> KFNDTLFGEMLHGYNNRTQHVNQGQVFQMTFRENNFIKDFPQLADGLLVIPLPVEEQCRGVLSEPLPDLQLLTGDIRYDEAMGYPMVQQWRVRSNLYRVKLSTITLAAGFTNVLKILTKESSREELLSFIQHYGSHYIAEALYGSELTCIIHFPSKKVQQQLWLQYQKETTELGSKKELKSMPFITYLSGLLTAQMLSDDQLISGVEIRCEEKGRCPSTCHLCRRPGKEQLSPTPVLLEINRVVPLYTLIQDNGTKEAFKSALMSSYWCS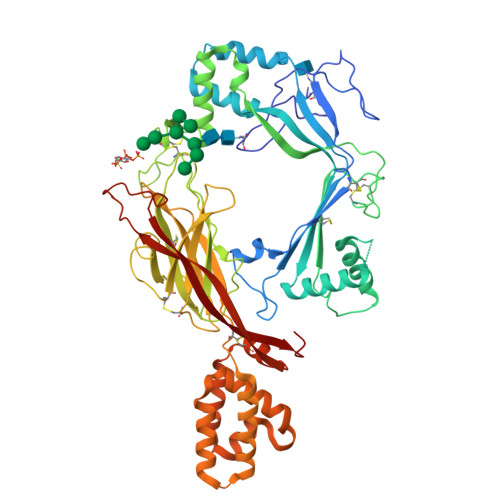GKGDVIDDWCRCDLSAFDANGLPNCSPLLQPVLRLSPTVEPSSTVVSLEWVDVQPAIGTKVSDYILQHKKVDEYTDTDLYTGEFLSFADDLLSGLGTSCVAAGRSHGEVPEVSIYSVIFKCLEPDGLYKFTLYAVDTRGRHSELSTVTLRTACPLVDDNKAEEIADKIYNLYNGYTSGKEQQMAYNTLMEVSASMLFRVQHHYNSHYEKFGDFVWRSEDELGPRKAHLILRRLERVSSHCSSLLRSAYIQSRVETVPYLFCRSEEVRPAGMVWYSILKDTKITCEEKMVSMARNTYGESKGR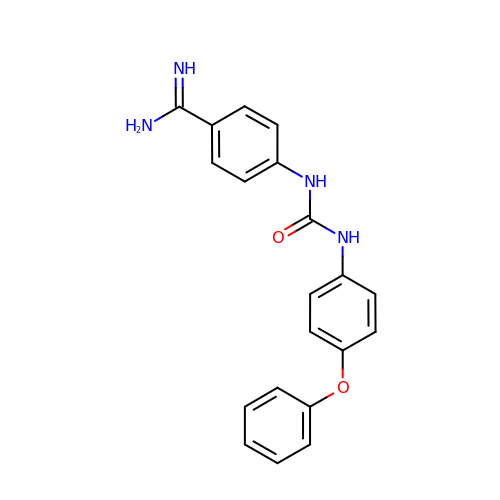1-(2-AMIDINOPHENYL)-3-(PHENOXYPHENYL)UREA | C20 H18 N4 O2 | ZHCAYBOLUMAUQX-UHFFFAOYSA-N>[2x]MNPDDIVVLVGRKKSGKSYLIKHYFIPVLKAHKISYIIDDHNLLRSGSEYSKFGYNATSLSDIVSKQYVVVYDRAKNDDFFEKLW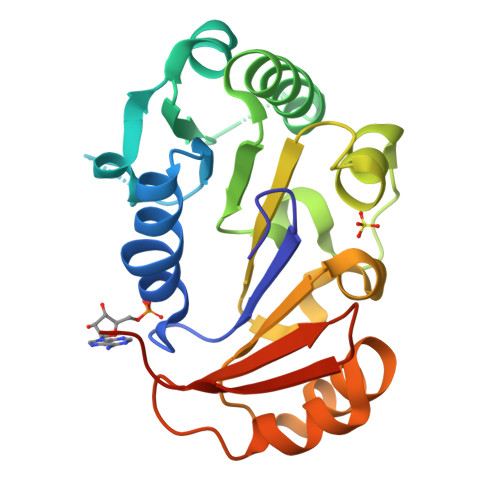QASKLHSKKYGTTVLIIDEAYYHFKYKQKVTPAIDEALHANRHAGLGLILSTQRVYDLMPIVYKQADLIIMFYTREPNELRWISKYISAEAAEKVKTLKQYHFLIYDVNSQTIKIHKPILEHHHHHH>DSRFGAKSISTIAESKRFPLHEMRDDVAFQIINDELYLDGNARQNLATFCQTWDDENVHKLMDLSINKNWIDKEEYPQSAAIDLRCVNMVADLWHAPAPKNGQAVGTNTIGSSEACMLGGMAMKWRWRKRMEAAGKPTDKPNLVCGPVQICWHKFARYWDVELREIPMRPGQLFMDPKRMIEACDENTIGVVPTFGVTYTGNYEFPQPLHDALDKFQADTGIDIDMHIDAASGGFLAPFVAPDIVWDFRLPRVKSISASGHKFGLAPLGCGWVIWRDEEALPQELVFNVDYLGGQIGTFAINFSRPAGQVIAQYYEFLRLGREGYTKVQNASYQVAAYLADEI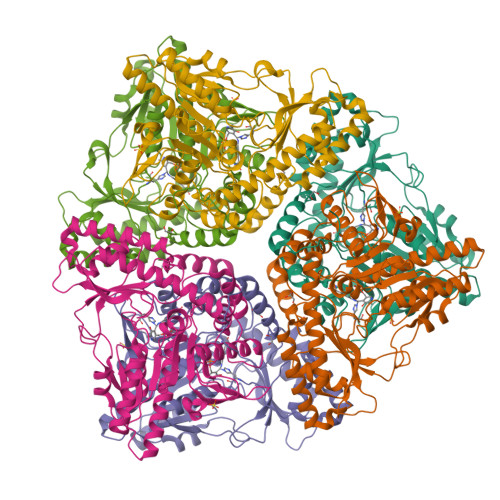AKLGPYEFICTGRPDEGIPAVCFKLKDGEDPGYTLYDLSERLRLRGWQVPAFTLGGEATDIVVMRIMCRRGFEMDFAELLLEDYKASLKYLSDHPKLQGIAQQNSFKHT[6x]>GSNLTSAPVPSTTTRSLTACPEESPLLVGPMLIEFNIPVDLKLVEQQNPKVKLGGRYTPMDCISPHKVAIIIPFRNRQEHLKYWLYYLHPILQRQQLDYGIYVINQAGESMFNRAKLLNVGFKEALKDYDYNC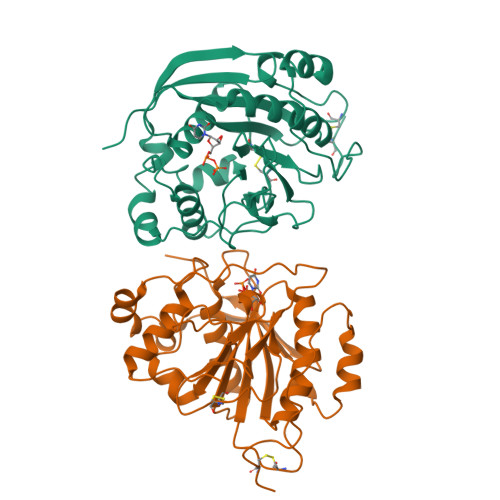FVFSDVDLIPMNDHNTYRCFSQPRHISVAMDKFGFSLPYVQYFGGVSALSKQQFLSINGFPNNYWGWGGEDDDIYNRLAFRGMSVSRPNAVIGKCRMIRHSRDKKNEPNPQRFDRIAHTKETMLSDGLNSLTYMVLEVQRYPLYTKITVDIGTPS[2x]> TPYDPLTLWTTPDPSPNCSLIQELDAKLTLCLTKNGSIVNGIVSLVGVK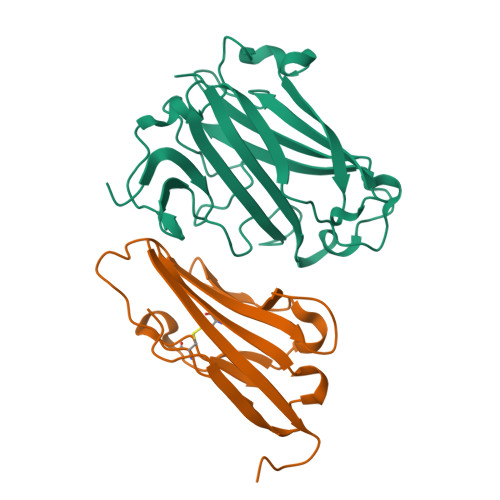GNLLNIQSTTTTVGVHLVFDEQGRLITSTPTALVPQASWGYRQGQSVSTNTVTNGLGFMPNVSAYPRPNASEAKSQMVSLTYLQGDTSKPITMKVAFNGITSLNGYSLTFMWSGLSNYINQPFSTPSCSFSYITQE;> GITTPEEMIEKAKGETAYLPCKFTLSPEDQGPLDIEWLISPADNQKVDQVIILYSGDKIYDDYYPDLKGRVHFTSNDLKSGDASINVTNLQLSDIGTYQCKVKKAPGVANKKIHLVVLVKPSGA3-methoxy-1,8-bis(oxidanyl)anthracene-9,10-dione | 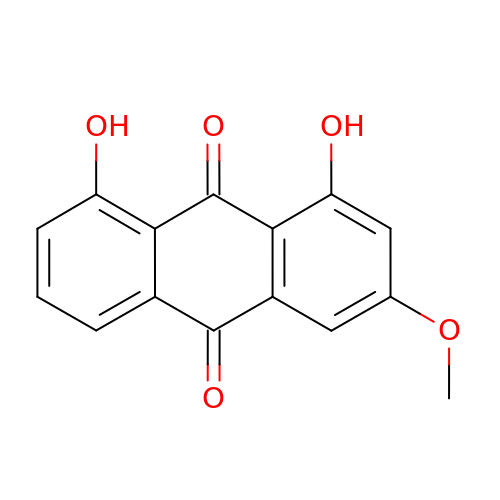C15 H10 O5 | ZMPLLBBFALVVAF-UHFFFAOYSA-N> MADKLFINALKKKFEESPEEKKTTFYTLGGWKQSERKTEFVNAGKEVAAKRGIPQYNPDIGTPLGQRVLMPYQVSTTDTYVEGDDLHFVNNAAMQQMWDDIRRTVIVGLNHAHAVIEKRLGKEVTPETITHYLETVNHAMPGAAVVQEHMVETHPALVADSYVKVFTGNDEIADEIDPAFVIDINKQFPEDQAETLKAEVGDGIWQVVRIPTIVSRTCDGATTSRWSAMQIGMSMISAYKQAAGEAATGDFAYAAKHAEVIHMGTYLPVRRARGENEPGGVPFGYLADICQSSRVNYEDPVRVSLDVVATGAMLYDQIWLGSYMSGGVGFTQYATAAYTDNILDDFTYFGKEYVEDKYGLCEAPNNMDTVLDVATEVTFYGLEQYEEYPALLEDQFGGSQRAAVVAAAAGCSTAFATGNAQTGLSGWYLSMYLHKEQHSRLGFYGYDLQDQCGASNVFSIRGDEGLPLELRGPNYPNYAMNVGHQGEYAGISQAPHAARGDAFVFNPLVKIAFADDNLVFDFTNVRGEFAKGALREFEPAGER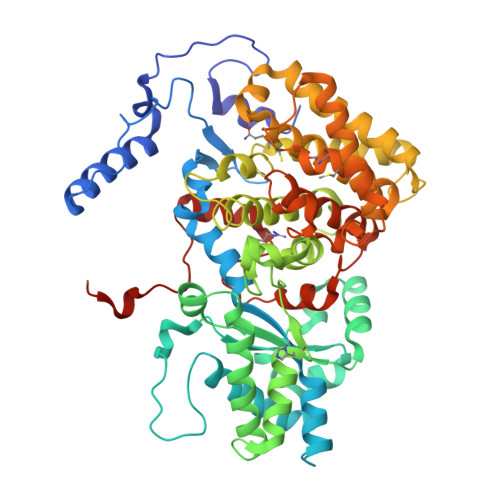ALITPAK>MHHHHHHGSDDDDKRPEAKSAQPADGWKGERPRSEEDNELNLPNLAAAYSSILSSLGENPQRQGLLKTPWRAASAMQFFTKGYQETISDVLNDAIFDEDHDEMVIVKDIDMFSMCEHHLVPFVGKVHIGYLPNKQVLGLSKLARIVEIYSRRLQVQERLTKQIAVAITEALRPAGVGVVVEATHMCMVMRGVQKMNSKTVTSTMLGVFREDPKTREEFLTLIRS[10x]

Guanosine triphosphate (GTP) cyclohydrolase I (GCH1) (EC:3.5.4.16) catalyzes the conversion of GTP to dihydroneopterin triphosphate (H2NTP). This reaction is the first and rate-limiting step involved in the de novo synthesis of tetrahydrobiopterin (BH4). The effects of GFRP on GCH1 occur via formation of heteromeric protein complexes between GCH1 and GFRP, which are dependent on the intracellular concentrations of the effector molecules phenylalanine or BH4. GCH1−GFRP complexes consist of one GCH1 decamer flanked by two pentameric GFRP complexes.

AXSP0056BS (cpd-1) was identified as an allosteric GCH1 inhibitor in an enzymatic assay with half maximal inhibitory concentration (IC50) values of 4 µM. From one cocrystallization campaign, surprisingly, we obtained two independent structures of allosterically inhibited GCH1: one fully inhibited form (xtal_GCH1_allosteric) with all allosteric sites occupied by inhibitor, and a partially inhibited form (xtal_GCH1_allosteric), in which only two of five allosteric pockets in each GCH1 pentamer were occupied with cpd-1. The same degree of disorder seen for the inhibitory cryo-EM structure was observed for the xtal_GCH1_allosteric structure, while region A is ordered and F122 is in a defined closed state in xtal_GCH1+active. We do not see any major differences between the cryo-EM structure of the BH4−GFRP-inhibited GCH1 and the X-ray structure of cpd-1−inhibited GCH1. In particular, the quaternary structural changes in region C are replicated in the X-ray structure, namely, the shift of the central α-helices. The shrinking of the β-barrel radius is even more pronounced, and the radius of the β-barrel decreases by 5 Å, when compared to apo GCH1. Thus, the major trigger for the large change in quaternary structure and compaction of the GCH1 interior is binding of ligands into the inhibitory allosteric pocket, independent from association of GFRP. Region B consisting of residues 213 to 222 is only weakly defined in the electron densities in all structures without an active site ligand bound (xtal_GCH1, EM_GCH1+hGFRP+allosteric, and xtal_GCH1+allosteric).> GSPAKIKIVAPLESALIPGGETYQLRCDIMSTPAATIHWKFNGKLIQGSNELNVEEKLLNFGKAIVDTGIVASILTIQCPSAENSGTYSCVGYNGHQTIETVAEVEIEGEASGCRSNHKSAP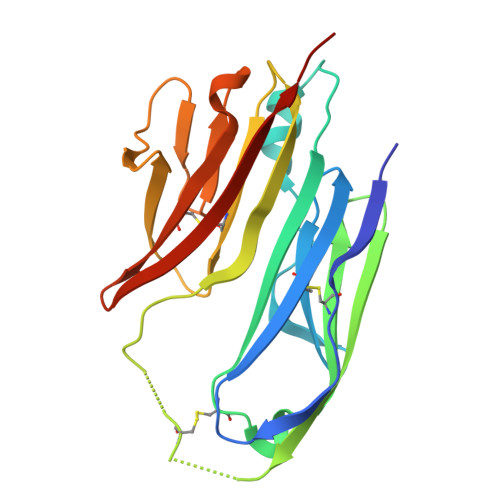EIVFWTDSRFEMTGNVATLVCRANQQVDWVWMSNDELVKNNDKFTVLSNGDLVIKNIVWDDMGTYTCIARNQFGEARQETFLYPTAHHHHHH3,7-BIS(DIMETHYLAMINO)PHENOTHIAZIN-5-IUM | 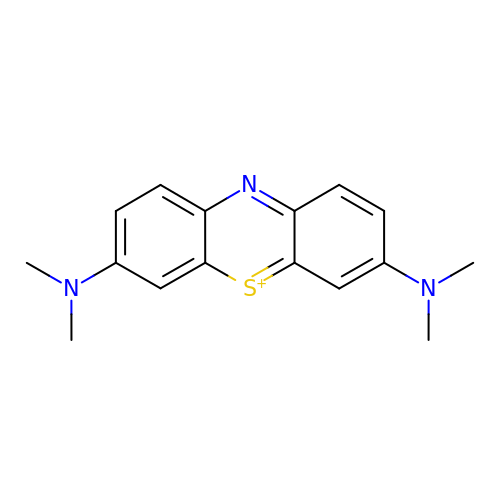C16 H18 N3 S | RBTBFTRPCNLSDE-UHFFFAOYSA-N Survival of motor neuron (SMN) functions in diverse biological pathways via recognition of symmetric dimethylarginine (Rme2s) on proteins by its Tudor domain, and deficiency of SMN leads to spinal muscular atrophy. Here we report a potent and selective antagonist with a 4-iminopyridine scaffold targeting the Tudor domain of SMN. In order to understand the structural basis of compound 1 recognition by these reader proteins, we determined the crystal structures of compound 1 in complex with SMN, TDRD3 and UHRF1, respectively. In this study, we identified some low micromolar antagonists with a 4-iminopyridine scaffold targeting the Tudor domain of SMN, and compound 1 shows >4-fold selectivity over other tested methyllysine or methylarginine binding domains.

To explore if we could identify more potent compounds than compound 1, we procured commercially available analogs of compound 1 that include single, double and triple ring molecules and measured their binding affinities to SMN or UHRF1, respectively. SMN bound to all the four triple-ring compounds with affinities between 2.6 and 31 μM. The four triple-ring compounds have a 4-iminopyridine scaffold in common, and none of them is more potent than the original hit. However, the positive binding results of 1-substituted pyridine cores to SMN presented here could confirm that N132 does interact with the imino group and substituents on the pyridine nitrogen would point away from the Tudor domain, as larger 1-substituents would otherwise clash inside the aromatic cage. Indeed, our crystal structure of SMN in complex with compound 4 also confirms that the imino group of compound 4 forms a hydrogen bond with N132. In addition to triple-ring compounds 1 to 4, SMN also bound to two of twelve double-ring compounds, compounds 5 and 6. Both compounds retain the imino group, which pinpoints the importance of the imino group-mediated hydrogen bond in the compound binding and is consistent with our crystal structures of SMN in complex with compounds 1, 4, and 6.

> KKNTAASLQQWKVGDKCSAIWSEDGCIYPATIASIDFKRETCVVVYTGYGNREEQNLSDLLSPICE>SNAMIRDTATNTTQTQAAPQQAPAQQFTQAPQEKPMQSTQSQPTPSYAGTGGINSQFTRSGNVQGGDARASEALTVFTRLKEQAVAQQDLADDFSILRFDRDQHQVGWSSLVIAKQISLNGQPVIAVRPLILPNNSIELPKRKTNIVNGMQTDVIESDIDVGTVFSAQYFNRLSTYVQNTLGKPGAKVVLAGPFPIPADLVLKDSELQLRNLLIKSVNACDDILALHSGERPFT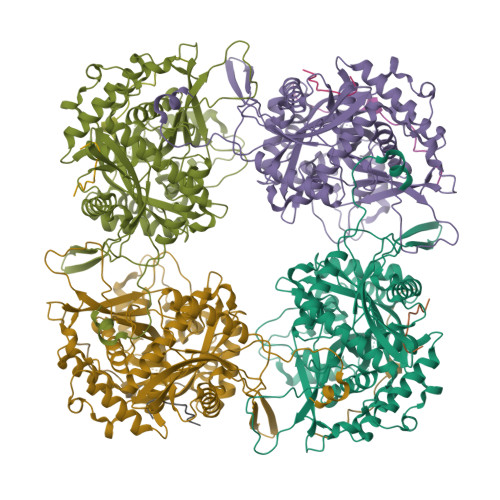IAGLKGQQGETLAAKVDIRTQPLHDTVGNPIRADIVVTTQRVRRNGQQENEFYETDVKLNQVAMFTNLERTPQAQAQTLFPNQQQVATPAPWVASVVITDVRNADGIQANTPEMYWFALSNAFRSTHGHAWARPFLPMTGVAKDMKDIGALGWMSALRNRIDTKAANFDDAQFGQLMLSQVQPNPVFQIDLNRMGETAQMDSLQLDAAGGPNAQKAAATIIRQINNLGGGGFERFFDHTTQPILERTGQVIDLGNWFDGDEKRDRRDLDNLAALNAAEGNENEFWGFYGAQLNPNLHPDLRNRQSRNYDRQYLGSTVTYTGKAERCTYNAKFIEALDRYLAEAGLQITMDNTSVLNSGQRFMGNSVIGNNMVSGQAQVHSAYAGTQGFNTQYQTGPSSFY[12x]> MTHIDKIQALAFSIGKKMQTELLEQMQATGLTPPQFYILKILDHYGASRATTLAKKMYVKPSAITVMIDRLIDQELVERYHDKDDRRVVIIELTKKGKARVEEAMTARNEHIAKYFSHLELQEREDLLRLFEKLETI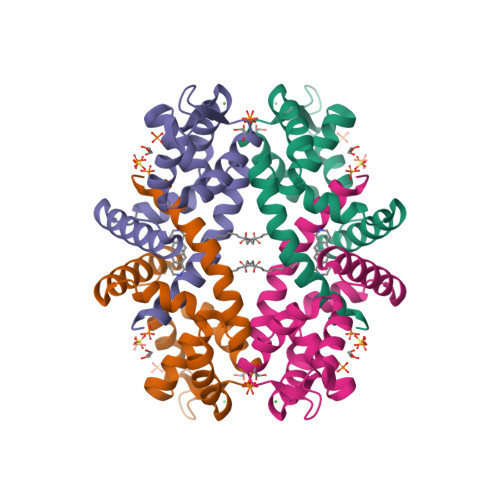ICGTQ> MAGKKGQKKSGLGNHGKNSDMDVEDRLQAVVLTDSYETRFMPLTAVKPRCLLPLANVPLIEYTLEFLAKAGVHEVFLICSSHANQINDYIENSKWNLPWSPFKITTIMSPEARCTGDVMRDLDNRGIITGDFILVSGDVLTNIDFSKMLEFHKKMHLQDKDHISTMCLSKASTYPKTRTIEPAAFVLDKSTSRCIYYQDLPLPSSREKTSIQIDPELLDNVDEFVIRNDLIDCRIDICTSHVPLIFQENFDYQSLRTDFVKGVISSDILGKHIYAYLTDEYAVRVESWQTYDTISQDFLGRWCYPLVLDSNIQDDQTYSYESRHIYKEKDVVLAQSCKIGKCTAIGSGTKIGEGTKIENSVIGRNCQIGENIRIKNSFIWDDCIIGNNSIIDHSLIASNATLGSNV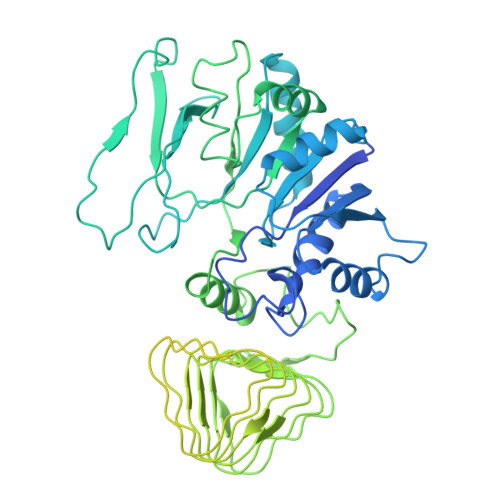RLNDGCIIGFNVKIDDNMDLDRNTKISASPLKNAGSRMYDNESNEQFDQDLDDQTLAVSIVGDKGVGYIYESEVSDDEDSSTEACKEINTLSNQLDELYLSDDSISSATKKTKKRRTMSVNSIYTDREEIDSEFEDEDFEKEGIATVERAMENNHDLDTALLELNTLRMSMNVTYHEVRIATITALLRRVYHFIATQTLGPKDAVVKVFNQWGLLFKRQAFDEEEYIDLMNIIMEKIVEQSFDKPDLILFSALVSLYDNDIIEEDVIYKWWDNVSTDPRYDEVKKLTVKWVEWLQNADEESSSEEE> MSLNREVKFRAWDKELNMMVYTKEQTGHIEYNTNPADTINIILNQDDYGYVFMQYTGLKDKNEKEIYEGDIIKKSNRSSNLYEIIYQDSIACFRCKVIKGDIKSFPCLNIGTVRNCEVIGNIYE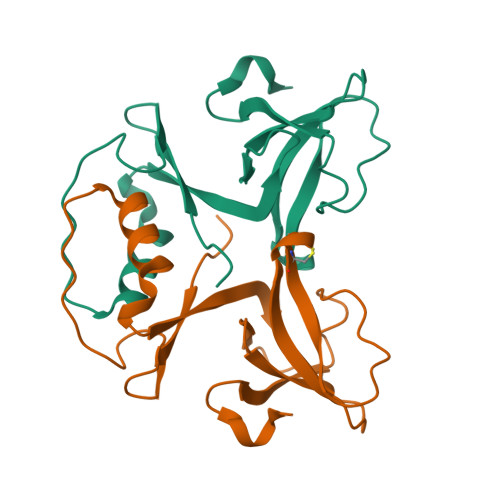NPELLEEEGHHHHHH> IFEERHLKYISQLGKGNFGSVELCRYDPLGDNTGALVAVKQLQHSGPDQQRDFQREIQILKALHSDFIVKYRGVSYGPGEPSLRLVMEYLPSGCLRDFLQRHRARLDASRLLLYSSQICKGMEYLGSRRCVHRDLAARNILVESEAHVKIADFGLAKLLPLDKDYYVVREPGQSPIFWYAPESLSDNIFSRQSDVWSFGVVLYELFTYCDKSCSPSAEFL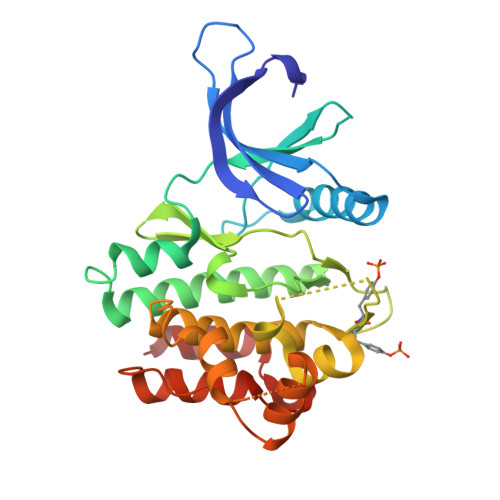RMMGCERDVPALSRLLELLEEGQRLPAPPACPAEVHELMKLCWAPSPQDRPSFSALGPQLDML> MLSDMSLIATL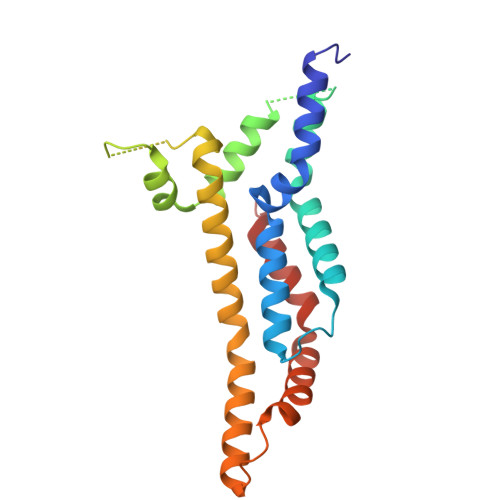SFFTLLPFLVAAGTCYIKFSIVFVMVRNALGLQQVPSNMTLNGIALIMALFVMKPIIEAGYENYLNGPQKFDTISDIVRFSDSGLMEYKQYLKKHTDLELARFFQRSEEENADLKSAENNDYSLFSLLPAYALSEIKDAFKIGFYLYLPFVVVDLVISSILLALGMMMMSPITISVPIKLVLFVALDGWGILSKALIEQYINIPA>SQIPASEQETLVRPKPLLLKLLKSVGAQKDTYTMKEVLYYLGQYIMTKRLYDEKQQHIVHCSNDLLGDLFGVPSFSVKEHRKI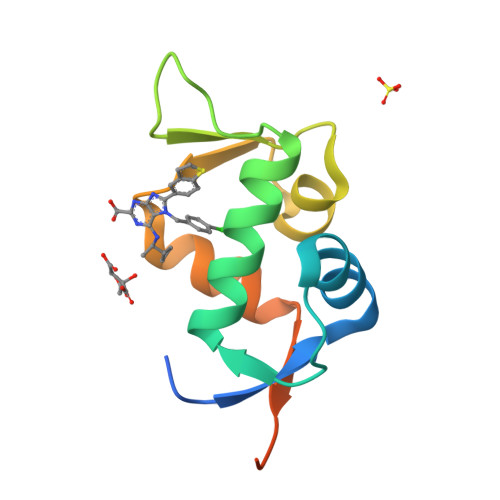YTMIYRNLVVVNQQESSDSGTSVSEN[2x]>MRWGYTSVQGFRDEMEDDIVIRSDAVDSFSYAAVFDGHAGSSSVKFLREELYKECVGALQAGSLLNGGDFAAIKEALIKAFESVDRNLLKWLEANGDEEDESGSTATVMIIRNDVSFIAHIGDSCAVLSRSGQIEELTDYHRPYGSSRAAIQEVKRVKEAGGWIVNGRICGDIAVSRAFGDIRFKTKKNDMLKKGVDEGRWSEKFVSRIEFKGDMVVATPDIFQVPLTSDVEFIILASDGLWDYMKSSDVVSYV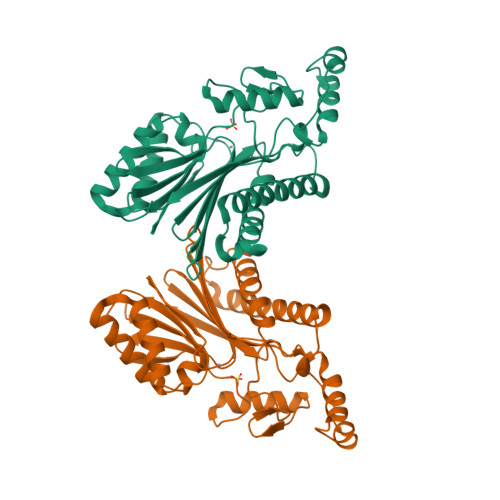RDQLRKHGNVQLACESLAQVALDRRSQDNISIIIADLGRTLEHHHHHH[2x]>GAMGSPGGSQQVEWVFIPVIKDVTYEFKVDNNDNITELYVNGNKLGPASSLE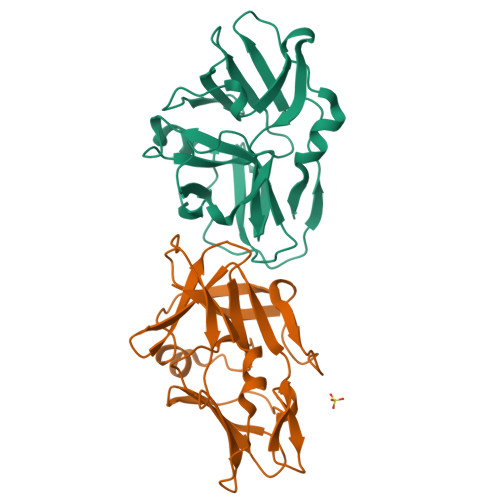MDFYFDVDVSNNQVRKFNNVFVLFGVIATKDSNKIKMQLTLNPCDFVRGFVFPSQDPSQLNNIFASNNKVSVSEKAFAILNRKKEGAVSSTINVYITQNTYTGNTKIEKIQQNTIIIEKNTGIVFKIPNDMLNIFRYSTT[4x]>WEYGDLHLFGPNQRPAPCYDPCEAVLVESIPEGLDFPNASTGNPSTSQAWLGLLAGAHSSLDIASFYWTLTNNDTHTQEPSAQQGEEVLRQLQTLAPKGVNVRIAVSKPSGPQPQADLQALLQSGAQVRMVDMQKLTHGVLHTKFWVVDQTHFYLGSANMDWRSLTQVKELGVVMYNCSCLARDLTKIFEAYWFLGQAGSSIPSTWPRFYDTRYNQETPMEICLNGTPALAYLASAPPPLCPSGRTPDLKALLNVVDNARSFIYVAVMNYLPTLEFSHPHRFWPAIDDGLRRATYERGVKVR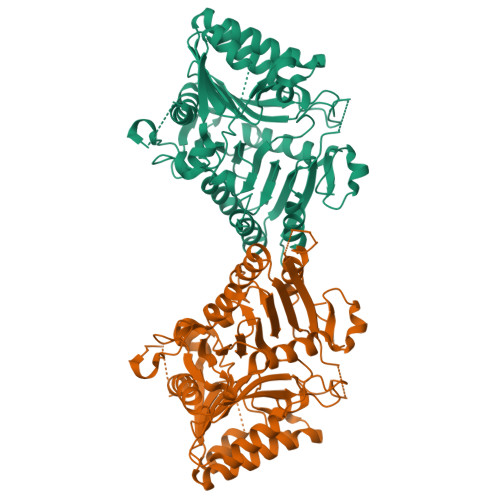LLISCWGHSEPSMRAFLLSLAALRDNHTHSDIQVKLFVVPADEAQARIPYARVNHNKYMVTERATYIGTSNWSGNYFTETAGTSLLVTQNGRGGLRSQLEAIFLRDWDSPYSHDLDTSADSVGNACRLL[2x]> GPDETLSLLADPYRFISRQCQRLGANAFESRFLLKKTNCLKGAKAAEIFYDTTRFEREGAMPVAIQKTLLGQGGVQGLDGETHRHRKQMFMGLMTPERVRALAQLFEAEWRRAVPGWTRKGEIVFYDELHEPLTRAVCAWAGVPLPDDEAGNRAGELRALFDAAGSASPRHLWSRLARRRVDAWAKRIIEGIRAGSIGSGSGTAAYAIAWHRDRHDDLLSPHVAAVELVNVLEPTVAIAVYITFVAHALQTCSGIRAALVQQPDYAELFVQEVRRFYPFFPAVVARASQDFEWEGMAFPEGRQVVLDLYGSNHDAATWADPQEFRPERFRAWDEDSFNFIPQG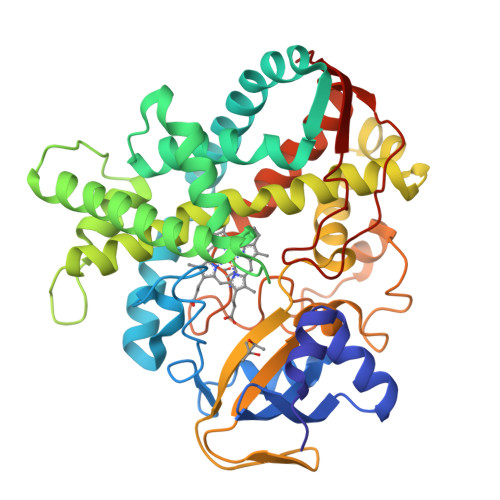GGDHYLGHRCPGEWIVLAIMKVAAHLLVNAMRYDVPDQDLSIDFARLPALPKSGFVMRNVHIGG>[2x]MEEEIILLDYWASMYGMRTRIALEEKKVKYEYREEDLSNKSPLLLQMNP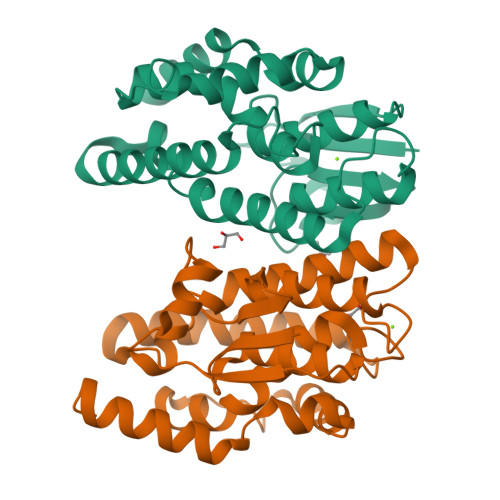IHKKIPVLIHEGKPICESIIQVQYIDELWPDTNPILPSDPYQRAQARFWADYIDKKTYVPCKALWSESGEKQEAAKIEFIEVLKTLDSELGDKYYFGGNEFGLVDIAFIGFYSWFRTYEEVANLSIVLEFPKLMAWAQRCLKRESVAKALPDSDKVLKSVSDHRKIILGID> GAMEGAGQMAELPTHYGTIIKTLRKYMKL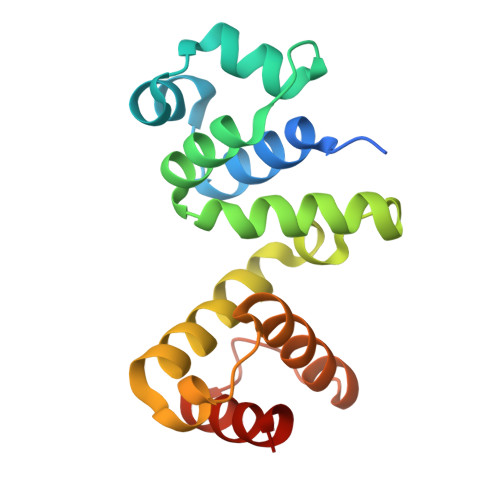TQSKLSERTGFSQNTISNHENGNRNIGVNEIEIYGKGLGIPSYILHRISDEFKEKGYSPTLNDFGKFDKMYSYVNKAYYNDGDIYYSSYDLYDETIKLLELLKESKINVNDIDYDYVLKLYKQILSTD SYRINGATE | C10 H12 O5 | 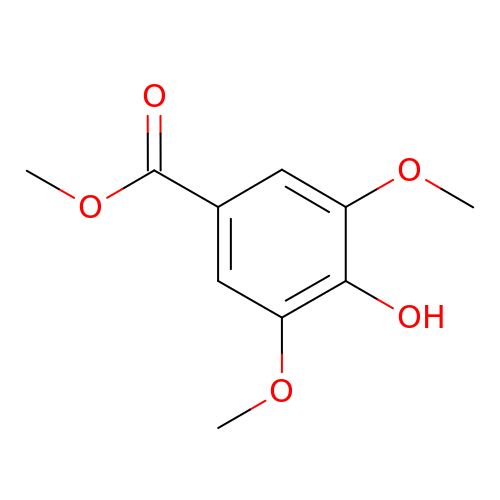ZMXJAEGJWHJMGX-UHFFFAOYSA-N> GAMSVPAIAPRRKRLADGLSV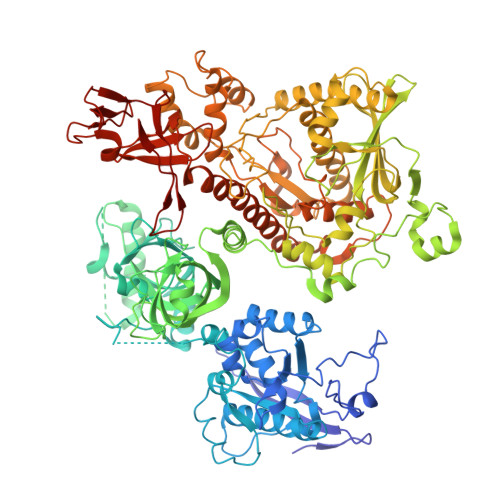TQKVFVRSRNGGATKIVREHYLRSDIPCLSRSCTKCPQIVVPDAQNELPKFILSDSPLELSAPIGKHYVVLDTNVVLQAIDLLENPNCFFDVIVPQIVLDEVRNKSYPVYTRLRTLCRDSDDHKRFIVFHNEFSEHTFVERLPNETINDRNNRAIRKTCQWYSEHLKPYDINVVLVTNDRLNREAATKEVESNIITKSLVQYIELLPNADDIRDSIPQMDSFDKDLERDTFSDFTFPEYYSTARVMGGLKNGVLYQGNIQISEYNFLEGSVSLPRFSKPVLIVGQKNLNRAFNGDQVIVELLPQSEWKAPSSIVLDSEHFDVNDNPDIEAGDDDDNNESSSNTTVISDKQRRLLAKDAMIAQRSKKIQPTAKVVYIQRRSWRQYVGQLAPSSVDPQSSSTQNVFVILMDKCLPKVRIRTRRAAELLDKRIVISIDSWPTTHKYPLGHFVRDLGTIESAQAETEALLLEHDVEYRPFSKKVLECLPAEGHDWKAPTKLDDPEAVSKDPLLTKRKDLRDKLICSIDPPGCVDINDALHAKKLPNGNWEVGVHIADVTHFVKPGTALDAEGAARGTSVYLVDKRIDMLPMLLGTDLCSLKPYVDRFAFSVIWELDDSANIVNVNFMKSVIRSREAFSYEQAQLRIDDKTQNDELTMGMRALLKLSVKLKQKRLEAGALNLASPEVKVHMDSETSDPNEVEIKKLLATNSLVEEFMLLANISVARKIYDAFPQTAMLRRHAAPPSTNFEILNEMLNTRKNMSISLESSKALADSLDRCVDPEDPYFNTLVRIMSTRCMMAAQYFYSGAYSYPDFRHYGLAVDIYTHFTSPIRRYCDVVAHRQLAGAIGYEPLSLTHRDKNKMDMICRNINRKHRNAQFAGRASIEYYVGQVMRNNESTETGYVIKVFNNGIVVLVPKFGVEGLIRLDNLTEDPNSAAFDEVEYKLTFVPTNSDKPRDVYVFDKVEVQVRSVMDPITSKRKAELLLK1-ethyl-3-[4-(hydroxymethyl)-5-(1H-pyrrol-2-yl)-1,3-thiazol-2-yl]urea | C11 H14 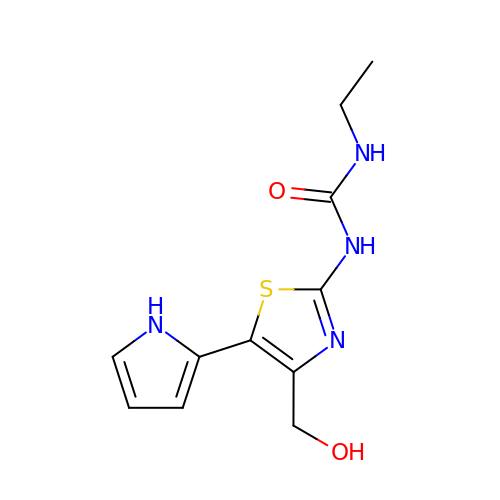N4 O2 S | YLSYQKDIZQYYGN-UHFFFAOYSA-N>[12x]GAMGIGKSPTGIQGFDELTLGGLPTGRPSLVCGSAGCGKTLFASTFLINGVRDHGEPGVFVTFEERPEDIVNNVASLGFELDKLIEEEKIAIEHIAVDPSEVAEIGDYDLEGLFLRLELAIDTVGAKRVVLDTIESLFSAFSNPAILRAEIRRLFDWLKERGLTTVITAERGDGALTRQGLEEYVSDCVILLDHRVENQISTRRLRIVKYRGTAHGTNEYPFLIDTDGFSVLPVSALGLLHQVHEERIASGVPDLDAMMAGGGFFRGSSILVSGVAGAGKSSLAAHFAAAACARGERAMYFSFEEAADQAVRNMRSLGLDLGRWRDAGLLRFMATRPTFYSLEMHLAVILREVMRFEPSVVVLDPISAFTESGDRLEVQSMLLRIVDFLKNRGITGIFTHLAHSQNEATTDAGLSSLMDGWVLMLNREVNGEFNRELYLLKARGMAHSNQVREFLMSDRGISLLPPHLGEGGALTGTARKAEEARLR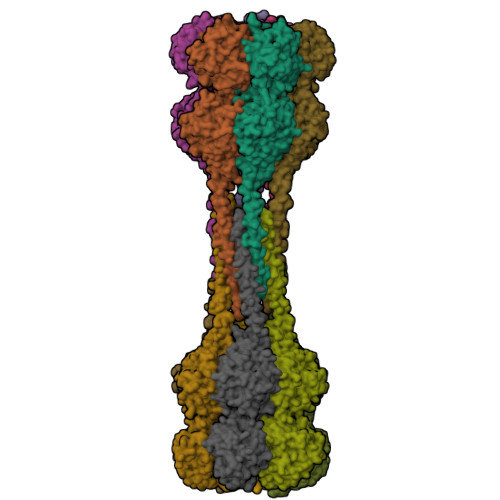RAEIERQTELGRLQQQIEQRRRRARAQIEALEAELQAEEIALKALVESESAHERQRLADADTLARSRGNERFADLLMNKGE>[9x]MIIDCHGHVSAPVELWAYKASLLAHRGSHGRGGVKVTDEQIIAAAHHKETWPDGHIELLHNHGTDMQLISPRPFQMMNSAKPARVVHWFCEEVNTLIHRQCTLIPEMFIPVAGLPQVAGEPIENVFAEMDRCVSMGFKGFLLNPDPYENGAEEAPPLGDRYWYPLYEKLCELDLPAHIHATGSQSERSPYSLHFINEETIATYNLCT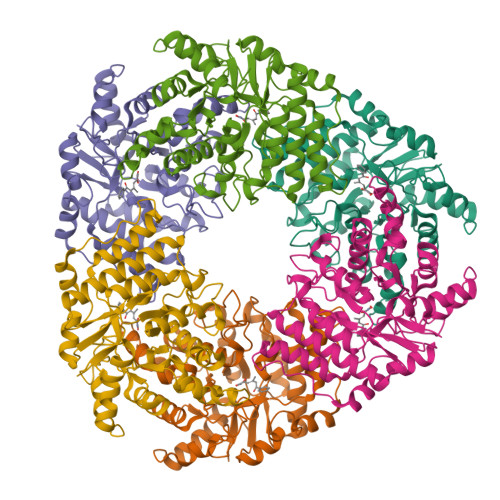SSVFDDFPQLKVVVSHGGGAIPYQLGRFESQSRRSKHLFSERMAKLYFDTVLYTEGALRLLIETVGPERCLFGSECPGVGSTIDPATGKQMDHIAPFIQKFDFLSDADKKLIFEDNARKVFNLEV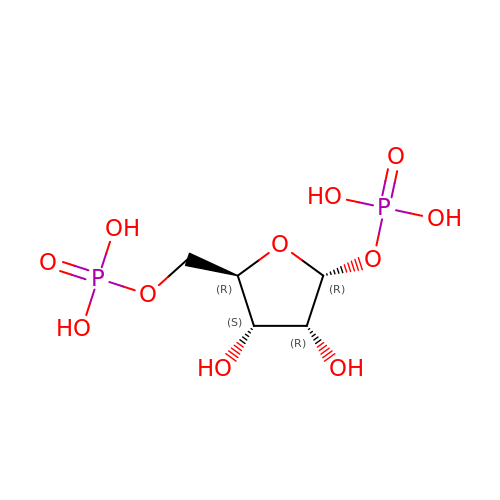1,5-di-O-phosphono-alpha-D-ribofuranose | C5 H12 O11 P2 | AAAFZMYJJHWUPN-TXICZTDVSA-N The structural and zinc-binding properties of PA4063, one of the periplasmic proteins expressed by Pseudomonas aeruginosa under zinc-deficient conditions, are presented. PA4063 has a noncanonical ferredoxin-like fold. Two zinc-binding sites with micromolar affinity are exposed and are located on the same face of the structure. Two histidine-rich loops, which are disordered in the apoprotein, contribute to zinc coordination in one of the sites. These findings strongly suggest a role for PA4063 in zinc trafficking, possibly acting as a metal chaperone or as a regulator of a transport system.

The structure of PA4063 in complex with zinc was solved by soaking crystals in zinc acetate solution since crystallization did not occur in presence of zinc. Soaking experiments were first performed with hexagonal crystals, despite their lower X-ray diffraction power, due to the poor reproducibility of the tetragonal crystals, leading to data collection to 3.3 Å resolution. Diffraction data were collected close to the absorption edge of zinc (λ = 1.27 Å) in order to unambiguously locate the metal. Two strong anomalous peaks were observed for each monomer (>9σ), revealing two binding sites, according to the ITC experiments, indicated as site a and site b. Site a is located on the flat surface of the β-sheet in correspondence with the histidine residues. The same mode of binding is detected in all three monomers of the hexagonal crystal: besides His124 and His126, the zinc ion binds to Glu87, likely as a monodentate ligand, and a water molecule, adopting a tetrahedral coordination geometry. Site b is about 20 Å from site a, on the edge of the β-sheet where the His-rich sequences are inserted. Notably, a few residues belonging to these sequences, which are disordered in apo PA4063, become structured and take part in zinc coordination, although some variability is present. As for site a, the coordination is tetrahedral and three donor groups are provided by one glutamate, Glu47, and two histidines, His16 and His18. The fourth donor was modelled as a water molecule in monomer A of the hexagonal crystal, while in monomers B and C, as well as in the tetragonal crystal, the electron-density map indicates His120 to be the donor. When evaluating the contribution of the His-rich sequences to the binding and the structural variation thus induced, it must be considered that the zinc-bound structure was obtained by soaking, thus the rearrangement could be influenced and limited by crystal packing.

>[3x]HDDHDHDHAHGSLGKHEHGVAQLNVALDGKTLELELDSPAMNLVGFEHAASTDADKAAVAKARAQLEKPLELFALPVTAGCSVASQELRSPLFGDKAPAHAHKEKAGHEHEHEHEHEHGHADIHAHYQLSCEKPELLKLLTLAEFFKRFPATQKIQVQLIGPDGQKGADLAPASAELKL> MANVEKMSVAVTPQQAAVMREAVEAGEYATASEIVREAVRDWLAKRELRHDDIRRLRQLWDEGKASGRPEPVDFDA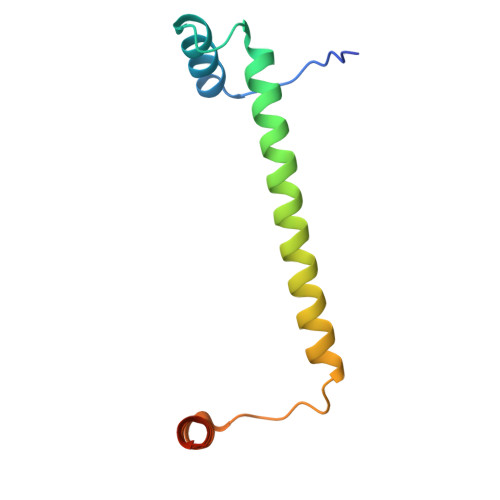LRKEARQKLTEVPPNGR> SNAMSEKPTSIKLVVVGDGAVGKTCLLISYSIRKFPEDYIPTVFDNYVVSLTAGTRQIQLALWDTAGLEEYDQLRPLSYSSASIFLICFSVTSSVSYDNVITKWHPEVIHFAPKVPIILVGTKLDTRNDPAIVKRLTEQGMTVINTAKG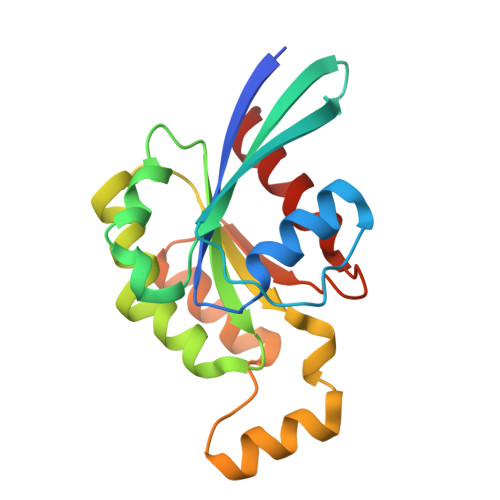EELKNRIKAVKYIECSAKTSENLKTVFDEAVKTVLMN The volume-regulated anion channel (VRAC), also called the volume-sensitive outwardly rectifying anion channel or volume-sensitive organic osmolyte-anion channel, is an anion channel activated upon cell swelling. The VRAC-mediated transport of chloride ions and small organic compounds, including osmolytes such as taurine or glutamate, drives water efflux to counteract cell swelling. Biochemical and biophysical analyses demonstrated that hetero-hexamers containing at least one LRRC8A isoform and at least one of the other four LRRC8 isoforms (LRRC8B-LRRC8E) form functional VRAC channels. The LRRC8D isoform is particularly interesting, because its incorporation into heteromers is requisite for the permeation of many organic substrates, independent of their electrical charge.

In this study, we present the 4.36 Å resolution cryo-EM structure of the human LRRC8D homo-hexamer, the largest isoform in the LRRC8 protein family, which is important to increase the permeability to organic substrates in VRAC. The final 3D map was reconstructed to an overall 4.36 Å resolution (local resolution of the transmembrane region is ~3.9 Å) with C2 symmetry imposed, and contained six subunits of HsLRRC8D (hereafter referred to as α to ζ subunits). Overall, HsLRRC8D adopts a homo-hexameric architecture composed of four regions: extracellular, TM, and intracellular regions in the N-terminal half of each subunit, and a leucine-rich repeat (LRR) region contained in the C-terminal half. The overall HsLRRC8D structure displays a twofold symmetric “dimer of trimers” arrangement; in other words, the structures of the α and δ subunits, those of the β and ε subunits, and those of the γ and ζ subunits are identical. Our HsLRRC8D structure revealed that, in addition to the threefold and sixfold symmetries, LRRC8 hexamers can form twofold symmetry. Notably, we discovered an additional N-terminal helix (NTH), which was not observed in the previously reported LRRC8A structures. It is formed by the N-terminal residues preceding the TM1 helix and protrudes into the channel pore, as in the previous structures of the connexin18,19,25 and innexin20,22 channels, which show weak homology to LRRC8 proteins. The NTH is formed by the Ala5 to Asn11 residues at the N-terminal region preceding the TM1 helix and closely interacts with the TM1 helix. In the HsLRRC8D structure, the Leu4, Val7, and Leu10 residues face the channel pore, whereas the Ala5, Ser9, and Asp12 residues face the TM1 helix. The sequence alignment predicted that the most constricted site is formed by the Phe143 residue, as its aromatic ring restricts the pore diameter to 11.5 Å.

>MFTLAEVASLNDIQPTYRILKPWWDVFMDYLAVVMLMVAIFAGTMQLTKDQVVCLPVLPSPVNSKAHTPPGNAEVTTNIPKMEAATNQDQDGRTTNDISFGTSAVTPDIPLRATYPRTDFALPNQEAKKEKKDPTGRKTNLDFQQYVFINQMCYHLALPWYSKYFPYLALIHTIILMVSSNFWFKYPKTCSKVEHFVSILGKCFESPWTTKALSETACEDSEENKQRITGAQTLPKHVSTSSDEGSPSASTPMINKTGFKFSAEKPVIEVPSMTILDKKDGEQAKALFEKVRKFRAHVEDSDLIYKLYVVQTVIKTAKFIFILCYTANFVNAISFEHVCKPKVEHLIGYEVFECTHNMAYMLKKLLISYISIICVYGFICLYTLFWLFRIPLKEYSFEKVREESSFSDIPDVKNDFAFLLHMVDQYDQLYSKRFGVFLSEVSENKLREISLNHEWTFEKLRQHISRNAQDKQELHLFMLSGVPDAVFDLTDLDVLKLELIPEAKIPAKISQMTNLQELHLCHCPAKVEQTAFSFLRDHLRCLHVKFTDVAEIPAWVYLLKNLRELYLIGNLNSENNKMIGLESLRELRHLKILHVKSNLTKVPSNITDVAPHLTKLVIHNDGTKLLVLNSLKKMMNVAELELQNCELERIPHAIFSLSNLQELDLKSNNIRTIEEIISFQHLKRLTCLKLWHNKIVTIPPSITHVKNLESLYFSNNKLESLPVAVFSLQKLRCLDVSYNNISMIPIEIGLLQNLQHLHITGNKVDILPKQLFKCIKLRTLNLGQNCITSLPEKVGQLSQLTQLELKGNCFDRLPAQLGQCRMLKKSGLVVEDHLFDTLPLEVKEALNQDINIPFANGIGTENLYFQ[6x]> MMLPKPGTYYLPWEVSAGQVPDGSTLRTFGRLCLYDMIQSRVTLMAQHGSDQHQVLVCTKLVEPFHAQVGSLYIVLGELQHQQDRGSVVKARVLTCVEGM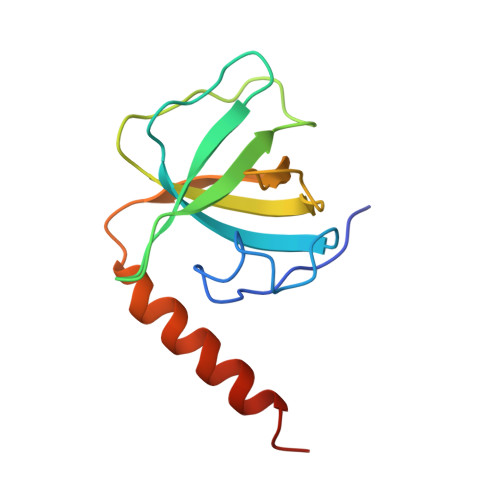NLPLLEQAIREQRLYKQERGGSQ>[2x]MKAPRILLSLLFSSLLLQAHALIPTDRKQRLTEHWEFIRQDMGSIWEVMRPITGAGKPETVPLWQKVTLPHCFNAEDAVDPDVNYYQGPGWYRTMLNIENPYTNGRTCLEFEGAGQKTEVYVYTTRIASHVGGYDEWKADITEAVEAFRRTPLCRERFGGKIPIAIRCDNSRDTEMIPSDMSDFNLYGGLYRYVNLVYTPAVHFEQIRIEATTDEKGKQGSISIDIAFGGLSGKEKKAKEFSLRVFSPEGKEVNSISSELTEISSYQISLKRPQLWSPHSPALYTCVAELIDNGDTLRTTQHFGFRHFRFEEK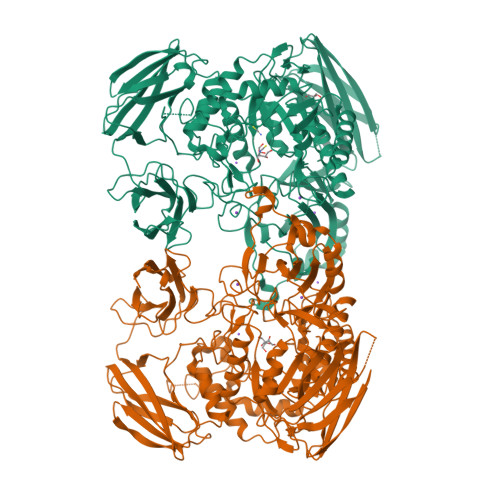GPFYLNGERLLLRGTHRHEDHAGVGAALTEEMMRTEMQQIKEMGANFIRLGHYQQSGIILRLCDELGLLVWEEIPWCRGGLGGESYKNQARRMLTNMIEQHRNHPSVILWGLGNENDWPGDFQTFEKDSIRAFMGELHDLAHRLDPTRSTAIRRCEFCKDIVDVYSPTIWAGWYGRRFRNYREMETAGINATTRFLHAEWGGDSHAGRHMEVNKETGRKGIDNFDIEAADRNGDWSESYIIRLFDWHLKEQETMPRLTGSLFWTFKDFSTPLRPDNPIPYVNQKGVVQRDGTPKESYYVFQSYWSSKPMLHIYGHSWPVRWGKPGEPKEILVYSNCPEVELFVNGVSQGRKKRNSQDFPAAGLRWNVPLREGNNKITATGYDGKLRLDDEIQQEYQTRTWGKPSRILLTQTAQDAETILVQAELIDENGIRCLDACQFIEFGCTDSEALLRNQGTAQGSRRIQAANGRASIRVNKQHAPVVVSASDSKRILKTALISVSGQ(3S)-3-(1H-indol-4-yl)-N7-methyl-N5-[(1R,5S)-3-oxabicyclo[3.1.0]hexan-6-yl]-2,3-dihydro-1-benzofuran-5,7-dicarboxamide 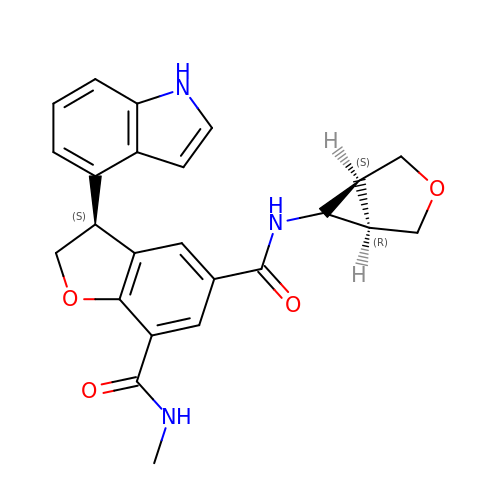| C24 H23 N3 O4 | MXVFNUYYLNWAFZ-CTAFRAEOSA-N>[2x]MELRAYTVLDALQPQLVAFLQTVSTGFMPMEQQASVLVEIAPGIAVNQLTDAALKATRCQPGLQIVERAYGLIEMHDDDQGQVRAAGDAMLAHLGAREADRLAPRVVSSQIITGIDGH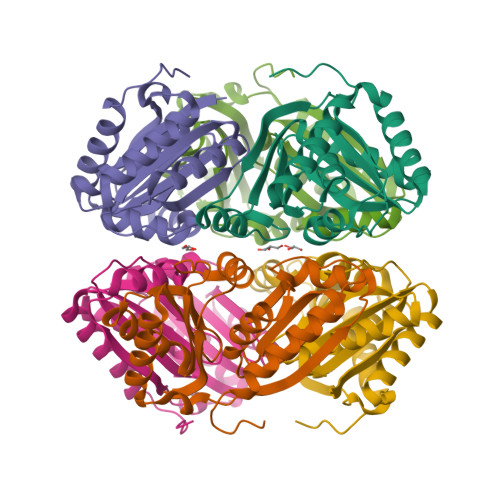QSQLINRMRHGDMIQAGQTLYILEVHPAGYAALAANEAEKAAPIKLLEVVTFGAFGRLWLGGGEAEIAEAARAAEGALAGLSGRDNRG>[4x]MALADISGYLDVLDSVRGFSYLENAREVLRSGEARCLGNPRSEPEYVKALYVIGASRIPVGDGCS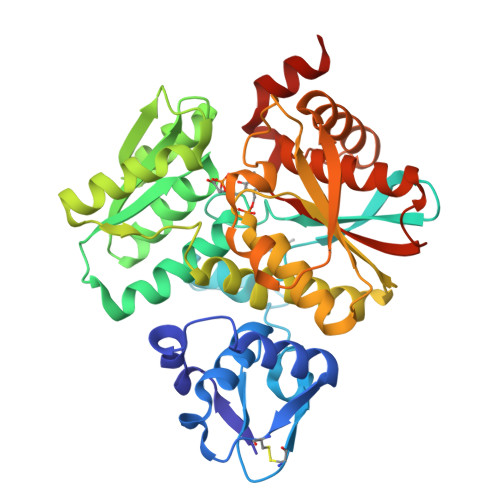HTLEELGVFDISVPGEMVFPSPLDFFERGKPTPLVRSRLQLPNGVRVWLKLEWYNPFSLSVADRPAVEIISRLSRRVEKGSLVADATSSNFGVALSAVARLYGYRARVYLPGAAEEFGKLLPRLLGAQVIVDPEAPSTVHLLPRVMKDSKNEGFVHVNQYYNDANFEAHMRGTAREIFVQSRRGGLALRGVAGSLGTSGHMSAAAFYLQSVDPSIRAVLVQPAQGDSIPGIARVETGMLWINMLDISYTLAEVTLEEAMEAVVEVARSDGLVIGPSGGAAVKALAKKAAEGDLEPGDYVVVVPDTGFKYLSLVQNALEGAGDSV> 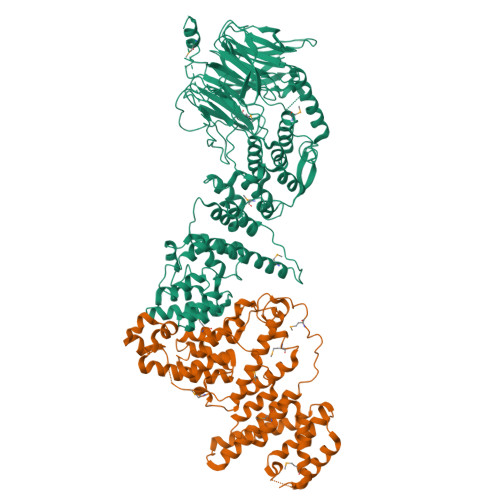MVVIANAHNELIHDAVLDYYGKRLATCSSDKTIKIFEVEGETHKLIDTLTGHEGPVWRVDWAHPKFGTILASCSYDGKVLIWKEENGRWSQIAVHAVHSASVNSVQWAPHEYGPLLLVASSDGKVSVVEFKENGTTSPIIIDAHAIGVNSASWAPATIEEDGEHNGTKESRKFVTGGADNLVKIWKYNSDAQTYVLESTLEGHSDWVRDVAWSPTVLLRSYLASVSQDRTCIIWTQDNEQGPWKKTLLKEEKFPDVLWRASWSLSGNVLALSGGDNKVTLWKENLEGKWEPAGEVHQGGGGSGGGGATSKEFDGPCQNEIDLLFSECNDEIDNAKLIMKERRFTASYTFAKFSTGSMLLTKDIVGKSGVSIKRLPTELQRKFLFDDVYLDKEIEKVTIEARKSNPYPQISESSLLFKDALDYMEKTSSDYNLWKLSSILFDPVSYPYKTDNDQVKMALLKKERHCRLTSWIVSQIGPEIEEKIRNSSNEIEQIFLYLLLNDVVRASKLAIESKNGHLSVLISYLGSNDPRIRDLAELQLQKWSTGGCSIDKNISKIYKLLSGSPFEGLFSLKELESEFSWLCLLNLTLCYGQIDEYSLESLVQSHLDKFSLPYDDPIGVIFQLYAANENTEKLYKEVRQRTNALDVQFCWYLIQTLRFNGTRVFSKETSDEATFAFAAQLEFAQLHGHSLFVSCFLNDDKAAEDTIKRLVMREITLLRASTNDHILNRLKIPSQLIFNAQALKDRYEGNYLSE;> GSMELSPTYQTERFTKFSDTLKEFKIEQNNEQNPIDPFNIIREFRSAAGQLALDLANSGDESNVISSKDWELEARFWHLVELLLVFRNADLDLDEMELHPYNSRGLFEKKLMQDNKQLYQIWIVMVWLKENTYVMERPKNVPTSKWLNSITSGGLKSCDLDFPLRENTNVLDVKDKEEDHIFFKYIYELILAGAIDEALEEAKLSDNISICMILCGIQEYLNPVIDTQIANEFNTQQGIKKHSLWRRTVYSLSQQAGLDPYERAIYSYLSGAIPNQEVLQYSDWESDLHIHLNQILQTEIENYLLENNQVGTDELILPLPSHALTVQEVLNRVASRHPSESEHPIRVLMASVILDSLPSVIHSSVEMLLDVVKGTEASNDIIDKPYLLRIVTHLAICLDIINPGSVEEVDKSKLITTYISLLKLQG>MKTPTIPTLLGPDGMTSLREYAGYHGGGSGFGGQLRSWNPPSESVDAALLPNFTRGNARADDLVRNNGYAANAIQLHQDHIVGSFFRLSHRPSWRYLGIGEEEARAFSREVEAAWKEFAEDDCCCIDVERKRTFTMMIREGVAMHAFNGELFVQATWDTSSSRLFRTQFRMVSPKRISNPNNTGDSRNCRAGVQINDSGAALGYYVSEDGYPGWMPQKWTWIPRELPGGRASFIHVFEPVEDGQTRGANVFYSVMEQMKMLDTLQNTQLQSAIVKAMYAATIESELDTQSAMDFILGANSQEQRERLTGWIGEIAAYYAAAPVRLGGAKVPHLMPGDSLNLQTAQDTDNGYSVFEQSLLRYIAAGLGVSYEQLSRNYAQMSYSTARASANESWAYFMGRRKFVASRQASQMFLCWLEEAIVRRVVTLPSKARFSFQEARSAWGNCDWIGSGRMAIDGLKEVQEAVMLIEAGLSTYEKECAKRGDDYQEIFAQQVRETMERRAAGLKPPAWAAAAFESGLRQSTEEEKSDSRAA[12x];>MTRQEELAAARAAL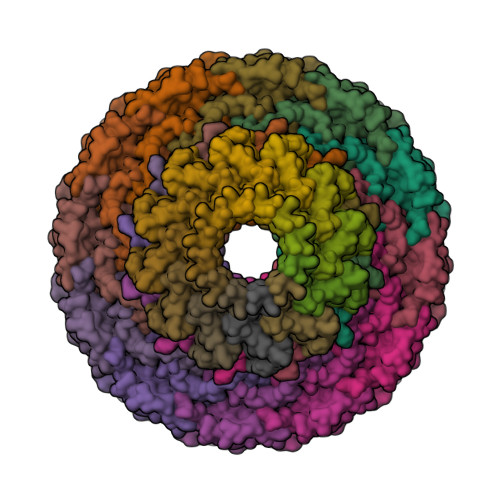HDLMTGKRVATVQKDGRRVEFTATSVSDLKKYIAELEVQTGMTQRRRGPAGFYV[12x]>MHHHHHHSSGRENLYFQGAIIKNVKVPDNYEIKHLIGRGSYGYVYLAYDKNANKNVAIKKVNRMFEDLIDCKRILREITILNRLKSDYIIRLHDLIIPEDLLKFDELYIVLEIADSDLKKLFKTPIFLTEQHVKTILYNLLLGEKFIHESGIIHRDLKPANCLLNQDCSVKICDFGLARTINSDKDIHIVNDLEEKEENEEPGPHNKNLKKQLTSHVVTRWYRAPELILLQENYTNSIDIWSTGCIFAELLNMMKSHINNPTNRFPLFPGSSCFPLSPDHNSKKVHEKSNRDQLNIIFNVIGTPPEEDLKCITKQEVIKYIKLFPTRDGIDLSKKYSSISKEGIDLLESMLRFNA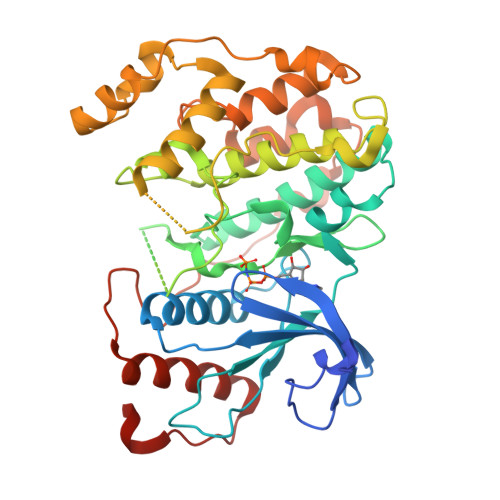QKRITIDKALSHPYLKDVRKENLENFSTEKIILPFDDWMVLSETQLRYIFLKEIQSFHADLIIPAKLNIHQKSF[2x]> 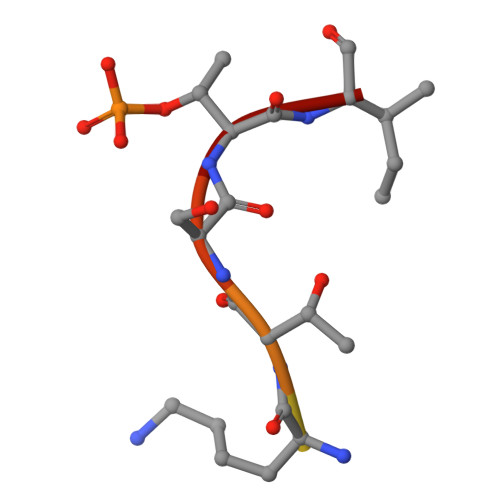FSQHKTSTI> MSNQQGPEDNNLEDDMAYLPADHPLLAKLQIDLTKQLTDEHERVDQKLIEIDANLKKLEKTKEDIGVRLYSVQQQLAENQMNFEQAHENYNWVQKLRIEAEQKLKTESEVYDAKKKELEELRKKYLKAQDELSKLTRTLYQINEFNQQMKGQIINTKTNTYRAEENVVNLEAQKKKQDLLIDTMNEEIKRQTEQKTILTAQLISQKEETEQAKQILKEAHLEMQKIIASKKNLLERWQKSLMTMQRMDNALQAIKEALKGQQELNLQIGTELNGVNAEIRKETEIQESLEGKNKKFDYEKDYLQKKYNELQEEKSKLEAQINLLTQSLRQTETEAGRAEIDKRNIEDQMNLIETNIMKLHTETKKLWEDLVHQKSEHTTIEKTATNLNKQANQISIEIEDKSVELENLLNEIARVKIDQLNTLSQIEVLENKRREVIKEREEKEITVATYEVQIRQGHDLNEKKQHEVGRLNREH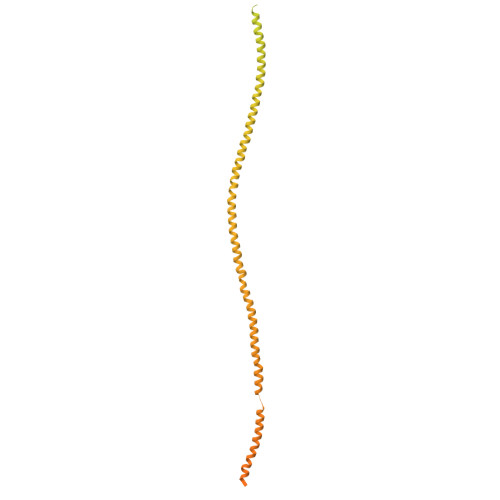DKLSSVQSDMSRGPLEAKRNNLIRKTQELGKENDLMQREWIKKQTLLVTQNNRLNKIEEDVSQLKTKQTILEQKKLRLNNNYRIYEKDIREIQNALKNLRNEMNKLNDAIYRNKEKQQKLDNENFNIKSEFVEKLKELEKESVKLEVEIDRLKEEKADLLAEIVESERQILLWERKIQLEKEMQDALDPTVGQTEIQELKREIHRMELRLDDLRKKQEAIIAEMERAVYKRETIQLKYMNKDKTFSNSNSMSQKSSSISAASDNSAQITKKIAQLKTTLNQTTRNAEQMEKAIKNKKIELDDLNAQIEGNNDNLQKLESDCYNKNIELTKHKLERSTNILSISCMQNKAKKLEDLVAGKARLSVPEATLMTKYEELRDKNQEIKEALQKLCDDAPQYVEVLNYLIDLNVGDDDEDQEQ> SGSAEIGTGFPFDPHYVEVLGERMHYVDVGPRDGTPVLFLHGNPTSSYVWRNIIPHVAPTHRCIAPDLIGMGKSDKPDLGYFFDDHVRFMDAFIEALGLEEVVLVIHDWGSALGFHWAKRNPERVKGIAFMEFIRPIPTWDEWPEFARETFQAFRTTD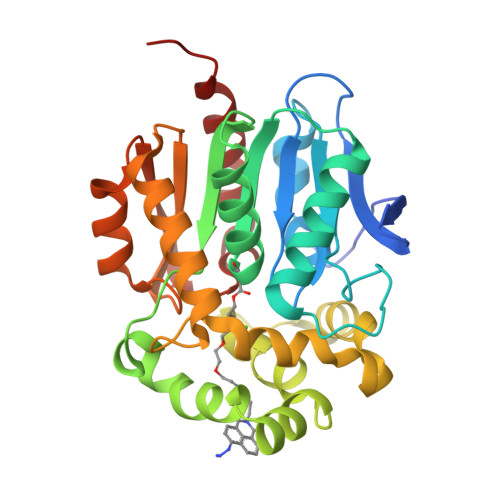VGRKLIIDQNVFIEGTLPCGVVRPLTEVEMDHYREPFLNPVDREPLWRFPNELPIAGEPANIVALVEEYMDWLHQSPVPKLLFWGTPGVLIPPAEAARLAKSLPNCKAVDIGPGLNLLQEDNPDLIGSEIARWLSTLEISG> GPLGSVWQLISKVLARHFSAADASRVLEQLQRDY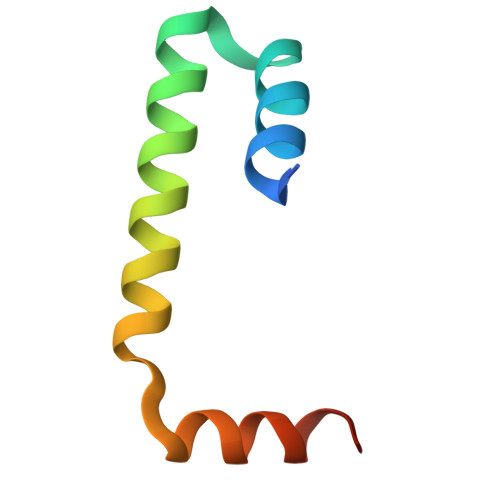ERSLSRLTLDDIERLASRFLHPEV>SKNKSMRGKKKSIFETYMSKEDVSEGLKRGTLIQGVLRINPKKFHEAFIPSPDGDRDIFIDGVVARNRALNGDLVVVKLLPEDQWKAVKPESNDKEIEATYEADIPEEGCGDDSDSEDRHGNTSGLVDGVKKLSILSEKSLQKSAKVVYILEKKHSRAATGILKLLADKNSDLFKKYALFSPSDHRVPRIYVPLKDCPQDFMTRPKDFANTLFICRIIDWKEDCNFALGQLAKSLGQAGEIEPETEGILTEYGVDFSDFSSEVLECLPQSLPWTIPPDEVGKRRDLRKDCIFTIDPSTARDLNDALACRRLTDGTFEVGVHIADVSYFVPEGSSLDKVAAERATSVYLVQKVVPMLPRLLCEELCSLNPMTDKLTFSVIWKLTPEGKILEEWFGRTIIRSCTKLSYDHAQSMIENPTEKIPEEELPPISPEHSVEEVHQAVLNLHSIAKQLRRQRFVDGALRLDQLKLAFTLDHETGLPQGCHIYEYRDSNKLVEEFMLLANMAVAHKIFRTFPEQALLRRHPPPQTKM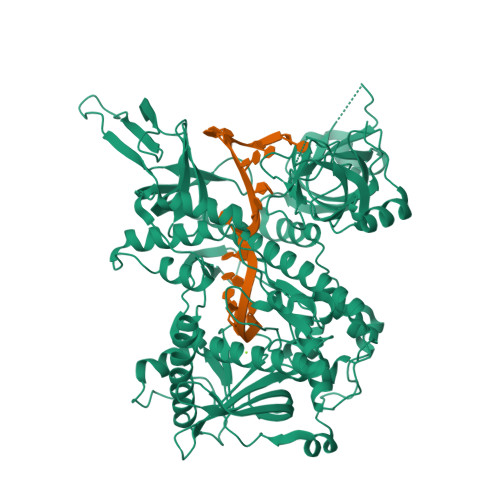LSDLVEFCDQMGLPMDVSSAGALNKSLTKTFGDDKYSLARKEVLTNMYSRPMQMALYFCSGMLQDQEQFRHYALNVPLYTHFTSPIRRFADVIVHRLLAAALGYSEQPDVEPDTLQKQADHCNDRRMASKRVQELSIGLFFAVLVKESGPLESEAMVMGVLNQAFDVLVLRFGVQKRIYCNALALRSYSFQKVGKKPELTLVWEPDDLEEEPTQQVITIFSLVDVVLQAEATALKYSAILK[2x]>[4x]G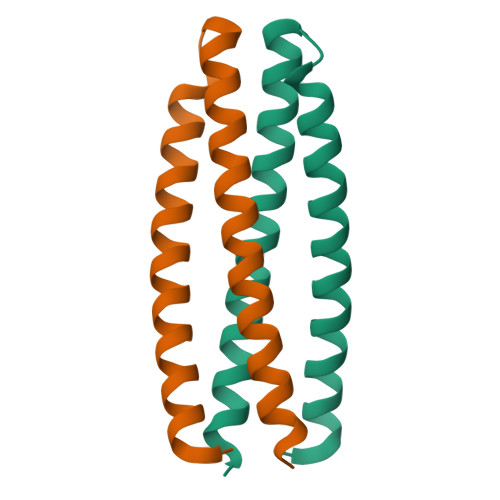SHMGTSDYIIEQIQRDQEEARKKVEEAEERLERVKEASKRGVSSDQLLDLIRELAEIIEELIRIIRRSNEAIKELIKNQS>GSVASVHASISGSSASSTSSTPEVKPLKSLLGDSAPTLHLNKGMAILFAVVARGTTILAKHAWCGGNFLEVTEQILAKIPSENNKLTYSHGNYLFHYICQDRIVYLCITDDDFERSRAFSFLNEVKKRFQTTYGS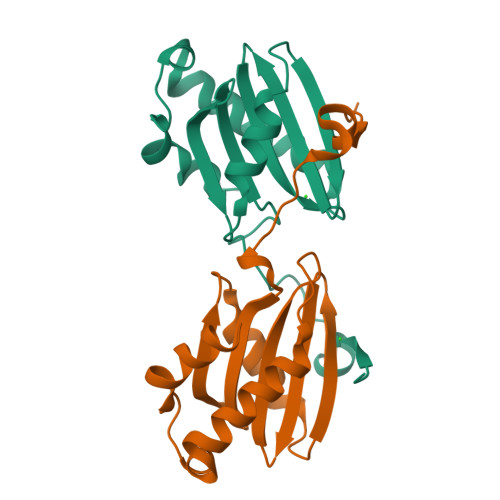RAQTALPYAMNSEFSSVLAAQLKHHSENHHHHHH[4x]> MIVAFCLYKYFPFGGLQRDF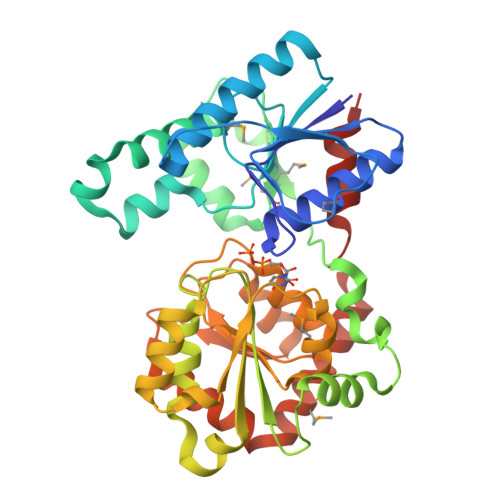MRIASTVAARGHHVRVYTQSWEGDCPKAFELIQVPVKSHTNHGRNAEYYAWVQNHLKEHPADRVVGFNKMPGLDVYFAADVCYAEKVAQEKGFLYRLTSRYRHYAAFERATFEQGKSTKLMMLTDKQIADFQKHYQTEPERFQILPPGIYPDRKYSEQIPNSREIYRQKNGIKEQQNLLLQVGSDFGRKGVDRSIEALASLPESLRHNTLLFVVGQDKPRKFEALAEKLGVRSNVHFFSGRNDVSELMAAADLLLHPAYQEAAGIVLLEAITAGLPVLTTAVCGYAHYIADANCGTVIAEPFSQEQLNEVLRKALTQSPLRMAWAENARHYADTQDLYSLPEKAADIITGGLDG3-[4-(3-oxidanylidenepropyl)piperazin-1-yl]propanal | C10 H18 N2 O2 | 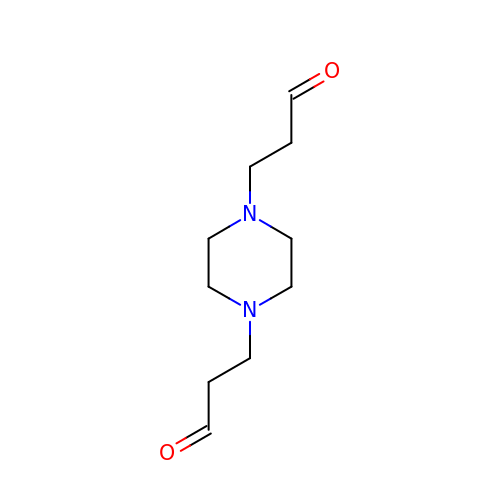YNICZMOQZCCMFE-UHFFFAOYSA-N FAM129B (family with sequence similarity 129, member B), also known as MINERVA (melanoma invasion by ERK), is a member of a small family of proteins that includes FAM129A and FAM129C, which are present only in vertebrates. Following the first identification of MINERVA as a target of ERK phosphorylation, several studies have reported that MINERVA is upregulated in many types of cancer, including breast, kidney, large intestine, lung and endometrial cancers as well as hematopoietic and central nervous system tumors. Overall, MINERVA modulates crosstalk among essential cellular signaling pathways for cell proliferation, invasion, and apoptosis. Sequence and secondary structure analyses of 746 amino acid-long MINERVA protein indicate a PH domain on the N-terminus (residues Asp66–Gly197) and a proline-rich region on the C-terminus (residues Asp575–Phe746) which contains the phosphorylatable serine residues.

Here, we report the first crystal structure of MINERVA lacking the C-terminal flexible region, which contains the PH domain and a helix bundle domain with a novel fold. The trypsin digestion greatly aided production of large single crystals of MINERVAΔC suitable for data collection, and hence was implemented for crystallizations of the native and SeMet-substituted MINERVAΔC. Using the SeMet-substituted structure as a molecular replacement (MR) model, we could successfully resolve the native MINERVAΔC structure for residues Gly2–Lys145 and Leu152–Arg560 at higher resolution. The structure of MINERVAΔC could be divided into two domains, the PH domain (residues Ile69–Asn196) and a helix bundle domain comprising the rest of the molecule, which exhibits a distorted L-shape where the PH domain is held at the corner of the helix bundle. The overall architecture of the helix bundle domain resembles no other known structure, as analyzed by Dali structural similarity search algorithm, suggesting that it is of a novel fold. The N-terminal PH domain is tightly held by the helix bundle domain that acts as a pincer-like scaffold, with a large contact area of 1573.4 Å2. The N-terminal PH domain adopts a typical fold of a PH domain containing a central curved antiparallel β-sheet (β5↑-β6↓-β7↑-β1↓-β2↑-β3↓-β4↑) followed by a C-terminal α-helix, α5. The spatial arrangement of the two domains allows the N-terminus of the protein to be located adjacent to the PH domain in proximity, presumably for cooperative action of myristoylated Gly2 residue and the PH domain for membrane localization of MINERVA. Surface representation of the protein reveals that MINERVA possesses a positively charged patch on its membrane-interacting face, which is mainly composed of positively charged residues Lys83, Lys84, Arg86, Lys104, Arg109, Arg114, Lys145, and Lys153 of the PH domain and Arg256, Lys258, and Lys260 of the helix bundle domain, presumably enabling stable interactions of MINERVA with the plasma membrane (top view).

> GDVLSTHLDDARRQHIAEKTGKILTEFLQFYEDQYGVALFNSMRHEIEGTGLPQAQLLWRKVPLDERIVFSGNLFQHQEDSKKWRNRFSLVPHNYGLVLYENKAAYERQVPPRAVINSAGYKILTSVDQYLELIGNSLPGTTAKSGSAPILKCPTQFPLILWHPYARHYYFCMMTEAEQDKWQAVLQDCIRHCNNGIPEDSKVEGPAFTDAIRMYRQSKELYGTWEMLCGNEVQILSNLVMEELGPELKAELGPRLKGKPQERQRQWIQISDAVYHMVYEQAKARFEEVLSKVQQVQPAMQAVIRTDMDQIITSKEHLASKIRAFILPKAEVCVRNHVQPYIPSILEALMVPTSQGFTEVRDVFFKEVTDMNLNVINEGGIDKLGEYMEKLSRLAYHPLKMQSCYEKMESLRLDGLQQRFDVSSTSVFKQRAQIHMREQMDNAVYTFETLLHQELGKGPTKEELCKSIQRVLERVLKKYDYDSSSVRKRFFREALLQISIPFLLKKLAPTCKSELPRFQELIFEDFARFILVENTYEEVVLQTVMKDILQAVKEAAVQR>MSLFGTTSGFGTSGTSMFGSATTDNHNPMKDIEVTSSPDDSIGCLSFSPPTLPGNFLIAGSWANDVRCWEVQDSGQTIPKAQQMHTGPVLDVCWSDDGSKVFTASCDKTAKMWDLSSNQAIQIAQHDAPVKTIHWIKAPNYSCVMTGSWDKTLKFWDTRSSNPMMVLQLPERCYCADVIYPMAVVATAERGLIVYQLENQPSEFRRIESPLKHQHRCVAIFKDKQNKPTGFALGSIEGRVAIHYINPPNPAKDNFTFKCHRSNGTNTSAPQDIYAVNGIAFHPVHGTLATVGSDGRFSFWDKDARTKLKTSEQLDQPISACCFNHNGNIFAYASSYDWSKGHEFYNPQKKNYIFLRNAAEELKPRNKK[2x];>[2x]MFNKSFGTPFGGGTGGFGTTSTFGQNTGFGTTSGGAFGTSAFGSSNNTGGLFGNSQTKPGGLFGTSSFSQPATSTSTGFGFGTSTGTANTLFGTASTGTSLFSSQNNAFAQNKPTGFGNFGTSTSSGGLFGTTNTTSNPFGSTSGSLFGPSSFTAAPTGTTIKFNPPTGTDTMVKAGVSTNISTKHQCITAMKEYESKSLEELRLEDYQANRKGPQNQVGAGTTTGLFGSSPATSSATGLFSSSTTNSGFAYGQNKTAFGTSTTGFGTNPGGLFGQQNQQTTSLFSKPFGQATTTQNTGFSFGNTSTIGQPSTNTMGLFGVTQASQPGGLFGTATNTSTGTAFGTGTGLFGQTNTGFGAVGSTLFGNNKLTTFGSSTTSAPSFGTTSGGLFGNKPTLTLGTNTNTSNFGFGTNTSGNSIFGSKPAPGTLGTGLGAGFGTALGAGQASLFGNNQPKIGGPLGTGAFGAPGFNTTTATLGFGAPQAPVALTDPNASAAQQAVLQQHINSLTYSPFGDSPLFRNPMSDPKKKEERLKPTNPAAQKALTTPTHYKLTPRPATRVRPKALQTTGTAKSHLFDGLDDDEPSLANGAFMPKKSIKKLVLKNLNNSNLFSPVNRDSENLASPSEYPENGERFSFLSKPVDENHQQDGDEDSLVSHFYTNPIAKPIPQTPESAGNKHSNSNSVDDTIVALNMRAALRNGLEGSSEETSFHDESLQDDREEIENNSYHMHPAGIILTKVGYYTIPSMDDLAKITNEKGECIVSDFTIGRKGYGSIYFEGDVNLTNLNLDDIVHIRRKEVVVYLDDNQKPPVGEGLNRKAEVTLDGVWPTDKTSRCLIKSPDRLADINYEGRLEAVSRKQGAQFKEYRPETGSWVFKVSHFSKYGLQDSDEEEEEHPSKTSTKKLKTAPLPPASQTTPLQMALNGKPAPPPQSQSPEVEQLGRVVELDSDMVDITQEPVLDTMLEESMPEDQEPVSASTHIASSLGINPHVLQIMKASLLTDEEDVDMALDQRFSRLPSKADTSQEICSPRLPISASHSSKTRSLVGGLLQSKFTSGAFLSPSVSVQECRTPRAASLMNIPSTSSWSVPPPLTSVFTMPSPAPEVPLKTVGTRRQLGLVPREKSVTYGKGKLLMDMALFMGRSFRVGWGPNWTLANSGEQLNGSHELENHQIADSMEFGFLPNPVAVKPLTESPFKVHLEKLSLRQRKPDEDMKLYQTPLELKLKHSTVHVDELCPLIVPNLGVAVIHDYADWVKEASGDLPEAQIVKHWSLTWTLCEALWGHLKELDSQLNEPREYIQILERRRAFSRWLSCTATPQIEEEVSLTQKNSPVEAVFSYLTGKRISEACSLAQQSGDHRLALLLSQFVGSQSVRELLTMQLVDWHQLQADSFIQDERLRIFALLAGKPVWQLSEKKQINVCSQLDWKRSLAIHLWYLLPPTASISRALSMYEEAFQNTSDSDRYACSPLPSYLEGSGCVIAEEQNSQTPLRDVCFHLLKLYSDRHYDLNQLLEPRSITADPLDYRLSWHLWEVLRALNYTHLSAQCEGVLQASYAGQLESEGLWEWAIFVLLHIDNSGIREKAVRELLTRHCQLLETPESWAKETFLTQKLRVPAKWIHEAKAVRAHMESDKHLEALCLFKAEHWNRCHKLIIRHLASDAIINENYDYLKGFLEDLAPPERSSLIQDWETSGLVYLDYIRVIEMLRHIQQVDCSGNDLEQLHIKVTSLCSRIEQIQCYSAKDRLAQSDMAKRVANLLRVVLSLHHPPDRTSDSTPDPQRVPLRLLAPHIGRLPMPEDYAMDELRSLTQSYLRELAVGSL;>MFHLVDFQVTIAEILLIIMRTFKVSIWNLDYIINLIIKNLSKSLTENKYSQLDEEQP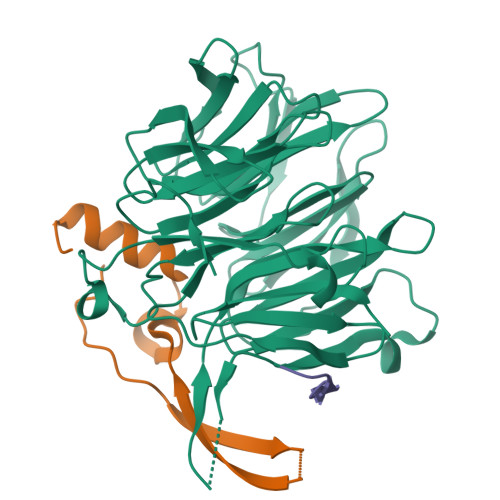MEID[2x]>[2x]MTHPSGEPVYADAVLNGWLTSMGLGVEYVRAEGNTVYYLDDEGREVPVLDHACGFGSLIFGHNHPEIIAHAKAALDAGTVVHAQLSRQPRANQISRILNDIMRRETGRDDRYNAIFANSGAEANEICMKHAELERQERITALFAEIDAELDTAREALTTGTATLDTASLPLVGGGAGDVDGVIADIHRHNDERRAERPLFLTLDGSFHGKLVGSIQLTQNEPWRTPFTALSSPARFLPADEPELIGKIVEDERRSVLTLSLDKD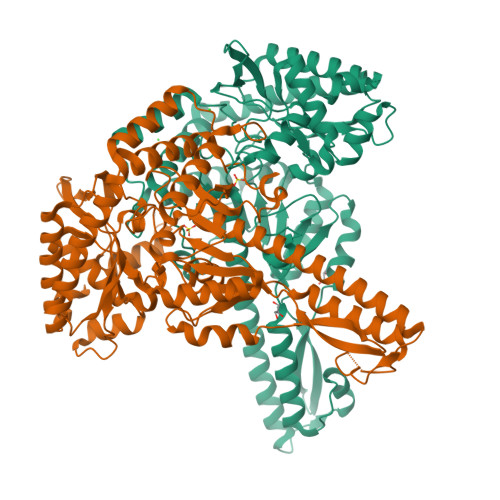TVRVVERDFPVVAAIFVEPVRGGSGMKTVTPELAEELHRLRDTLGCPLVVDEVQTGIGRTGAFFGSALLGIRGDYYTLAKAIGGGIVKNSVALIRQDRFLPAMEVIHSSTFAKDGLSASIALKVLEMVEADGGRVYQRVRERGQRLEAMLESVRADHSDVVSAVWGTGLMLALELRDQSNATSQAIREKAAHGFLGYVLAGFLLREHHIRVLPAGPRSGFLRFSPSLYITDEEIDRTETALRSLFTALRDQDGDRLVLS> QFQFTGI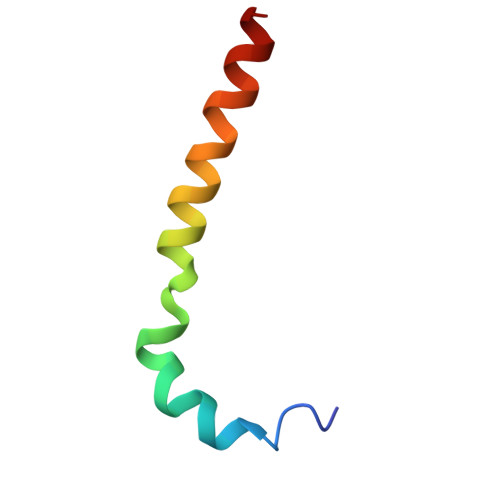KKYFNSYTLTGRMNCVLATYGGIALLVLYFKLRSK> MSADSSPLVGSTPTGYGTLTIGTSIDPLSSSVSSVRLSGYCGSPWRVIGYHVVVWMMAGIPLLLFRWKPLWGVRLRLRPCNLAHAETLVIEIRDKEDSSWQLFTVQVQTEAIGEGSLEPSPQSQAEDGRSQAAVGAVPEGAWKDTAQLHKSEEAVSVGQKRVLRYYLFQGQRYIWIETQQAFYQVSLLDHGRSCDDVHRSRHGLSLQDQMVRKAIYGPNVISIPVKSYPQLLVDEALNPYYGFQAFSIALWLADHYYWYALCIFLISSISICLSLYKTRKQSQTLRDMVKLSMRVCVCRPGGEEEWVDSSELVPGDCLVLPQEGGLMPCDAALVAGECMVNESSLTGESIPVLKTALPEGLGPYCAETHRRHTLFCGTLILQARAYVGPHVLAVVTRTGFCTAKGGLVSSILHPRPINFKFYKHSMKFVAALSVLALLGTIYSIFILYRNRVPLNEIVIRALDL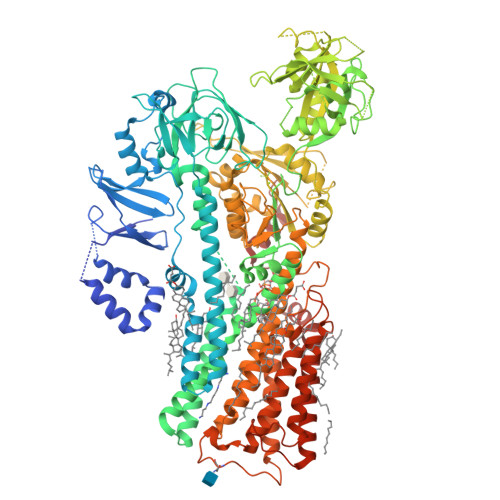VTVVVPPALPAAMTVCTLYAQSRLRRQGIFCIHPLRINLGGKLQLVCFDKTGTLTEDGLDVMGVVPLKGQAFLPLVPEPRRLPVGPLLRALATCHALSRLQDTPVGDPMDLKMVESTGWVLEEEPAADSAFGTQVLAVMRPPLWEPQLQAMEEPPVPVSVLHRFPFSSALQRMSVVVAWPGATQPEAYVKGSPELVAGLCNPETVPTDFAQMLQSYTAAGYRVVALASKPLPTVPSLEAAQQLTRDTVEGDLSLLGLLVMRNLLKPQTTPVIQALRRTRIRAVMVTGDNLQTAVTVARGCGMVAPQEHLIIVHATHPERGQPASLEFLPMESPTAVNGVKDPDQAASYTVEPDPRSRHLALSGPTFGIIVKHFPKLLPKVLVQGTVFARMAPEQKTELVCELQKLQYCVGMCGDGANDCGALKAADVGISLSQAEASVVSPFTSSMASIECVPMVIREGRCSLDTSFSVFKYMALYSLTQFISVLILYTINTNLGDLQFLAIDLVITTTVAVLMSRTGPALVLGRVRPPGALLSVPVLSSLLLQMVLVTGVQLGGYFLTLAQPWFVPLNRTVAAPDNLPNYENTVVFSLSSFQYLILAAAVSKGAPFRRPLYTNVPFLVALALLSSVLVGLVLVPGLLQGPLALRNITDTGFKLLLLGLVTLNFVGAFMLESVLDQCLPACLRRLRPKRASKKRFKQLERELAEQPWPPLPAGPLRSNSLEVLFQ>DVTPRRDAEYPPPEFLEAMKPLREICIKKTGVTEEAIIEFSD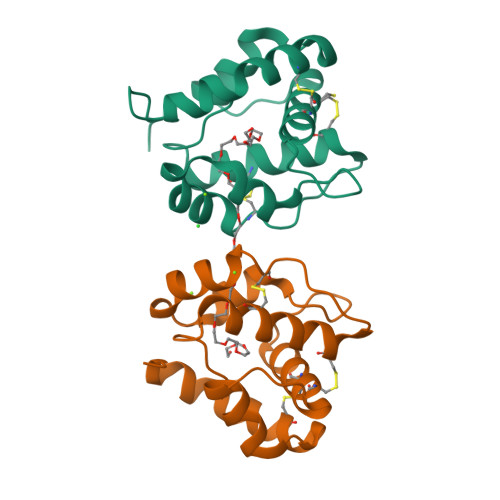GKVHEDENLKCYMNCLFHEAKVVDDTGHVHLEKLHDALPDSMHDIALHMGKRCLYPEGENLCEKAFWLHKCWKESDPKHYFLI[2x]> KQTARKST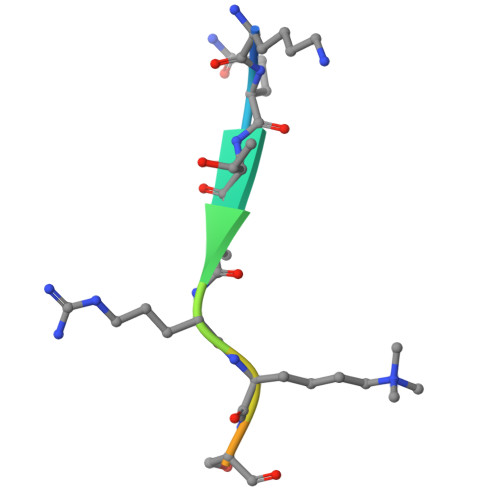GGK D-PROLINE | C5 H9 N O2 | 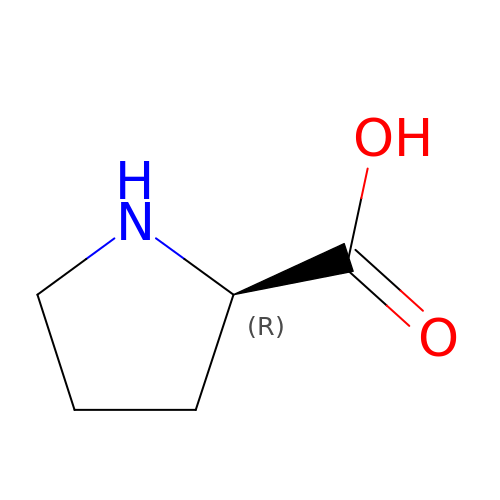ONIBWKKTOPOVIA-SCSAIBSYSA-N> MTDTTNSIKHVISPLARQTLQDRDLTRPVAGKRPIRLLPWLQVVKIGGRVMDRGADAILPLVEELRKLLPEHRLLILTGAGVRARHVFSVGLDLGLPVGSLAPLAASEAGQNGHILAAMLASEGVSYVEHPTVADQLAIHLSATRAVVGSAFPPYHHHEFPGSRIPPHRADTGAFLLADAFGAAGLTIVENVDGIYTADPNGPDRGQARFLPETSATDLAKSEGPLPVDRALLDVMATARHIERVQVVNGLVPGRLTAALRGEHVGTLIRTGVRPA;> MANSTAELEELLMQRSLTDPQLQAAAAAAADFRILPDATVIKIGGQSVIDRGRAAVYPLVDEIVAARKNHKLLIGTGAGTRARHLYSIAAGLGLPAGVLAQLGSSVADQNAAMLGQLLAKHGIPVVGGAGLSAVPLSLAEVNAVVFSGMPPYKLWMRPAAEGVIPPYRTDAGCFLLAEQFGCKQMIFVKDEDGLYTANPKTSKDATFIPRISVDEMKAKGLHDSILEFPVLDLLQSAQHVREVQVVNGLVPGN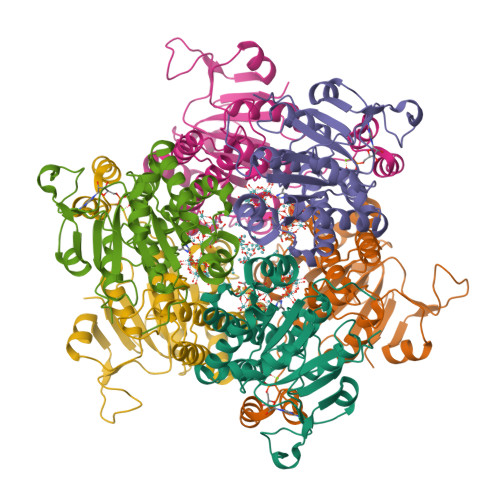LTRALAGEHVGTIITAS The attachment of myristate to the N-terminal glycine of certain proteins is largely a co-translational modification catalyzed by N-myristoyltransferase (NMT), and involved in protein membrane-localization. Using coenzyme A (CoA)-activated lipid, NMT transfers myristate to the substrate protein, after removal of the initiator methionine, in a predominantly co-translational process (Ritzefeld et al., 2017, Schlott et al., 2018). Pathogen NMT is a validated therapeutic target in numerous infectious diseases including malaria. PvNMT possesses 80% sequence identity and 93% similarity to PfNMT and is an excellent platform for structural studies, while to date PfNMT has proven intractable for X-ray crystallography.

Using these data, a structure-guided approach was used to identify compounds that can overcome resistance mediated by the G386E substitution, exploiting the differential binding mode of DDD85646. Analysis of the PvNMT[G386E] structure with either IMP-1002 or DDD85646 bound demonstrated that the positions of all three amino acids (E386, Y211, and H213) were influenced by the binding mode of the inhibitor. A preferred conformation (rotamer Y211a) was adopted in both the unliganded PvNMT[WT] and [G386E] enzymes, and, on binding of DDD85646 to PvNMT[WT], Y211 moved only slightly to rotamer Y211b when DDD85646 was bound to PvNMT[G386E]. Therefore, we measured the IC50 of DDD85646 with PvNMT[WT] and [G386E] enzyme and its EC50 with Pf3D7 [WT] and [G386E] parasite clones; compared with IMP-1002, the ratio of G386E/WT for DDD85646 was between 1 and 1.7 in both assays (CPM assay, IC50 ratio = 1.4 ± 0.35; growth assay, EC50 ratio = 1 ± 0.1), strengthening the hypothesis that DDD85646 binding is unaffected by G386E. This was supported by thermal shift data with DDD85646 that confirmed the difference in stabilization (ΔΔTm) between PvNMT[WT] and PvNMT[G386E] was only 3°C, significantly less than the >7.0°C in favor of WT observed for IMP-1002. Overall the minimal disruption of Y211 and H213 by DDD85646 binding results in the conserved affinity and binding mode for both WT and G386E variants, and these data together with minimally perturbed IC50, EC50, and thermal stability lead us to conclude that DDD85646 can break resistance in NMT[G386E] parasites. In combination with the shift in EC50, IC50, and thermal stability, the SPR data clearly show that DDD85646 can overcome resistance mediated by G386E. DDD85646 is insensitive to the resistance mechanism generated in response to IMP-1002 treatment, but at a cost of lower selectivity over HsNMT, because Y211 needs to move from the “in” Y211c rotamer occupancy, which provides improved selectivity over HsNMT (Yu et al., 2012), to the “out” Y211d rotamer, leaving room for G386E.

>[3x]MGSSHHHHHHSAALEVLFQGPDYKFWYTQPVPKINDEFNESVNEPFISDNKVEDVRKDEYKLPPGYSWYVCDVKDEKDRSEIYTLLTDNYVEDDDNIFRFNYSAEFLLWALTSPNYLKTWHIGVKYDASNKLIGFISAIPTDICIHKRTIKMAEVNFLCVHKTLRSKRLAPVLIKEITRRINLENIWQAIYTAGVYLPKPVSDARYYHRSINVKKLIEIGFSSLNSRLTMSRAIKLYRVEDTLNIKNMRLMKKKDVEGVHKLLGSYLEQFNLYAVFTKEEIAHWFLPIENVIYTYVNEENGKIKDMISFYSLPSQILGNDKYSTLNAAYSFYNVTTTATFKQLMQDAILLAKRNNFDVFNALEVMQNKSVFEDLKFGEGDESLKYYLYNWKCASFAPAHVGIVLL>[3x]GPAMLPISMSDEGDSFLVKDSLGENKIPKNPSKVVILDLGILDTFDALKLNDKVVGVPAKNLPKYLQQFKNKPSVGGVQQVDFEAINALKPDLIIISGRQSKFYDKLKEIAPTLFVGLDNANFLSSFENNVLSVAKLYGLEKEALEKISDIKNEIEKAKSIVDEDKKALIILTNSNKISAFGPQSRFGIIHDVLGINAVDENIKVGTLGKSINSEFILEKNPDYIFVVDRNVILGNKERAQGILDNALVAKTKAAQNKKIIYLDPEYWFLASGNGLESLKTMILEIKNAVK

The periplasmic binding protein (PBP) CeuE1 is an important component of the Fe(III) uptake system in Campylobacter jejuni, a commensal Gram-negative bacterium in the avian gut, but a common source of food poisoning in humans. CeuE, an integral part of the CeuBCDE ABC transporter of C. jejuni, is responsible for capturing Fe(III)-siderophore complexes in the periplasm for delivery to their respective inner membrane transporter. C. jejuni does not itself synthesize siderophores, but capitalizes on their secretion by other bacteria, such as E. coli. Here we report a combined solution and structural study of a series of synthetic tetradentate analogues of the enterobactin-derived bis(2, 3-dihydroxybenzoyl-L-Ser), to explore the ligand-binding promiscuity of CeuE, both wild type and with mutations of the Fe(III) binding residues H227 and Y288.

To probe the relative contributions of His227 and Tyr288 to Fe(III)-siderophore binding, site-directed mutagenesis was then used to replace the side chains of the two Fe(III)-coordinating amino acids with non-coordinating side chains of similar size. In addition, the double mutants H227L/Y288F and H227A/Y288F were created. All five mutants (Y288F, H227L, H227A, H227L/Y288F, H227A/Y288F) were crystallized in their apo form, and all structures are closely similar to that of wild type CeuE. However while there is clear electron density for the Y288F mutation in its three structures, H227L and H227A are located in a flexible loop region and there is generally no electron density to confirm their presence. Mutation of the Fe(III)-coordinating tyrosine led to a drastic drop in binding affinity in both the single (Y228F) and the double mutants (H227L/Y288F and H227A/Y288F), with Kd values above 1 μM. Site-directed mutagenesis of CeuE revealed that Y288 is essential for binding, as the binding affinity observed in the fluorescence titration experiments is far weaker for all mutants containing Y228F when compared to the wild type protein. This finding is confirmed by the lack of CD signal corresponding to the Λ-configuration when Fe-5-Lic is added to these mutants.>MGSSHHHHHHSSGLVPRGSHTGAGLRWKHTSSLKVANEPVLAFTQGSPERDALQKALKDLKGRMEAIPCVVGDEEVWTSDVQYQVSPFNHGHKV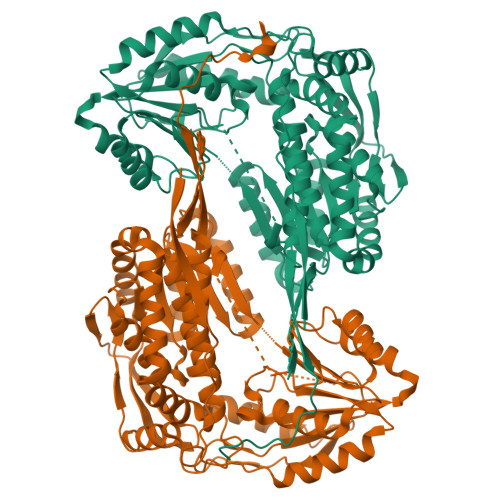AKFCYADKSLLNKAIEAALAARKEWDLKPIADRAQIFLKAADMLSGPRRAEILAKTMVGQGKTVIQAEIDAAAELIDFFRFNAKYAVELEGQQPISVPPSTNSTVYRGLEGFVAAISPFNFTAIGGNLAGAPALMGNVVLWKPSDTAMLASYAVYRILREAGLPPNIIQFVPADGPLFGDTVTSSEHLCGINFTGSVPTFKHLWKQVAQNLDRFHTFPRLAGECGGKNFHFVHRSADVESVVSGTLRSAFEYGGQKCSACLRLYVPHSLWPQIKGRLLEEHSRIKVGDPAEDFGTFFSAVIDAKSFARIKKWLEHARSSPSLTILAGGKCDDSVGYFVEPCIVESKDPQEPIMKEEIFGPVLSVYVYPDDKYKETLQLVDSTTSYGLTGAVFSQDKDVVQEATKVLRNAAGNFYINDKSTGSIVGQQPFGGARASGTNDKPGGPHYILRWTSPQVIKETHKPLGDWSYAYMQ[4x]>VGALAVVVWLWLWLWX[2x];>VGALAVVVWLFLWLWX[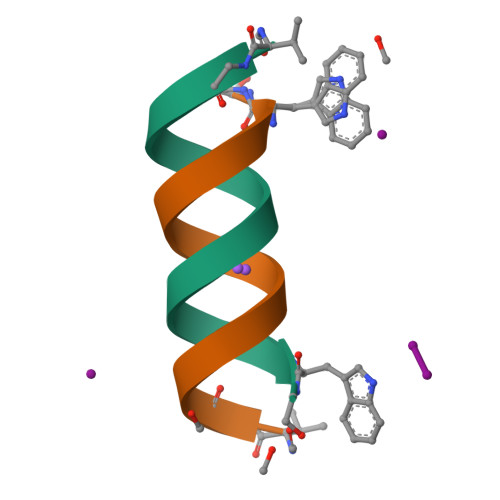2x]N-{3-[(4aR,7aR)-2-amino-4,4a,5,6-tetrahydro-7aH-furo[2,3-d][1,3]thiazin-7a-yl]-4-fluorophenyl}-5-bromopyridine-2-carboxamide | C18 H16 Br F N4 O2 S | 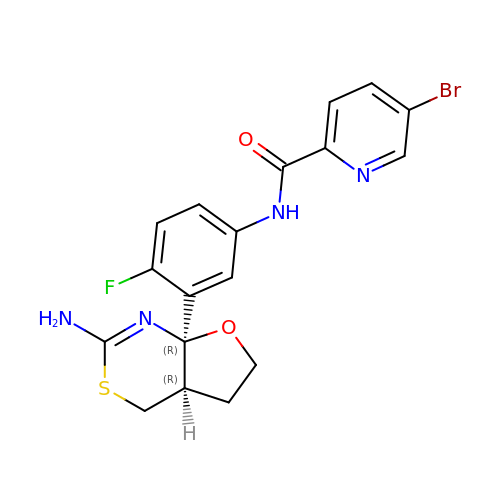DACRJCISVSMZQT-XTZNXHDOSA-N> QGMNTIESITADLHGLGVRPGDLIMVHASLKAVGPVEGGAASVVSALRAAVGSAGTLMGYASWDRSPYEETLNGARMDEELRRRWPPFDLATSGTYPGFGLLNRFLLEAPDARRSAHPDASMVAVGPLAATLTEPHRLGQALGEGSPLERFVGHGGKVLLLGAPLDSVTVLHYAEAIAPIPNKRRVTYEMPMLGPDGRVRWELAEDFDSNGILDCFAVDGKPDAVETIAKAYVELGRHREGIVGRAPSYLFEAQDIVSFGVTYLEQHFGAP

Here, we conduct a comprehensive functional analysis of the Antibiotic_NAT family of aminoglycoside acetyltransferases. AG resistance is primarily conferred by three classes of aminoglycoside-modifying enzymes (AMEs): phosphotransferases (APHs), nucleotidylyltransferases (ANTs), and acetyltransferases (AACs). AMEs permanently alter the AG substrate, preventing them from binding to their target, the A-site of the 16S rRNA in the bacterial ribosome. The fold typical of the Antibiotic_NAT family is evident in all structures, composed of 13 α-helices and 8 β-strands, and determined structures superpose with pairwise RMSD’s 0.8–1.0 Å between 197 to 266 matching Cα atoms.

The crystal structure of AAC(3)-IIb represents the first molecular image of enzymes with AAC(3)-II activity. Its structure superimposes with RMSD 0.7 Å over 221 Cɑ atoms with the previously characterized AAC(3)-VIa structure, consistent with our phylogenetic analysis placing both these enzymes in the group 4 of the Antibiotic_NAT family. Similarly to the AAC(3)-VIa enzyme, the minor subdomain loop of AAC(3)-IIb contains the conserved Asn208, which is predicted to clash with substituents at position 5 of the AG substrate, thereby explaining the lack of activity toward 4,5-disubstituted AGs. Other notable amino acids in the active site of AAC(3)-IIa that may restrict the size and positioning of AG substrates include Tyr66, positioned near the binding location of the double prime ring, and Phe97, positioned near the central 2-deoxystreptamine ring. Altogether, AAC(3)-IIb—like AAC(3)-VIa—harbors a more restricted active site, consistent with its limited AG specificity. The crystal structure of AAC(3)-IIb features an active site highly like that of AAC(3)-VIa, consistent with the 4,6-disubstituted specificity of Group 4 enzymes. Finally, AAC(3)-IIb was monomeric both in the crystal structure and in solution (not shown). Insert 3 forms a two-stranded antiparallel β-sheet while corresponding to a short α-helix found only in AAC(3)-IIb structure. Representatives of Antibiotic_NAT Groups 2 and 4 were the most restricted in their specificity, and this was reflected in more constrained and smaller active sites, as revealed by the structures of AAC(3)-IIb and AAC(3)-Xa.>[3x]GKKKVCYYYDGDIGNYYYGQGHPMKPHRIRMTHNLLLNYGLYRKMEIYRPHKATAEEMTKYHSDEYIKFLRSIRPDNMSEYSKQMQRFNVGEDCPVFDGLFEFCQLSTGGSVAGAVKLNRQQTDMAVNWAGGLHHAKKSEASGFCYVN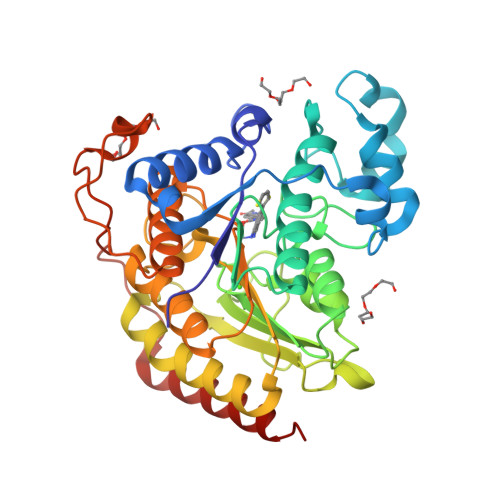DIVLAILELLKYHQRVLYIDIDIHHGDGVEEAFYTTDRVMTVSFHKYGEYFPGTGDLRDIGAGKGKYYAVNFPMRDGIDDESYGQIFKPIISKVMEMYQPSAVVLQCGADSLSGDRLGCFNLTVKGHAKCVEVVKTFNLPLLMLGGGGYTIRNVARCWTYETAVALDCEIPNELPYNDYFEYFGPDFKLHISPSNMTNQNTPEYMEKIKQRLFENLRMLPH> MFTKTGTTIVGVKYKGGVVICADTRSTSGPIVADKNCSKIHYISDNIQACGAGTSADITRVTRKASKVLSIFSKTYNRLPRVSHCVRTCQLHLHPYQGHISAALVVGGVDDTGAHLYDVYPHGSSNSVSYTALGSGSLAAISILEAGYKDMNREEAM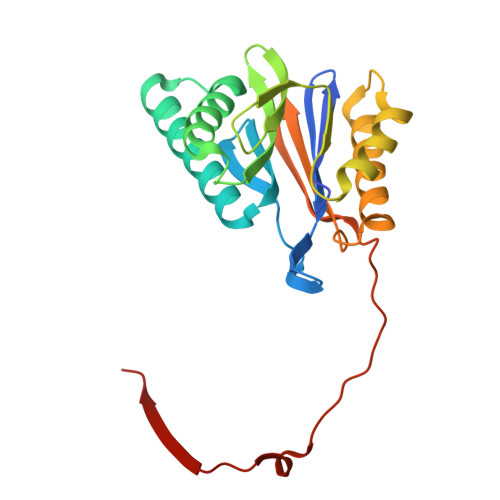ELACAAIEAGIMNDLYSGSNIDVCVISQEGREMFRNYKKVGVRNEVPKFQYPRSSVKILKEDIYKYIEEK>MKLDIKKTFSNRSDRVKGIDFHPTEPWVLTTLYSGRVEIWNYETQVEVRSIQVTETPVRAGKFIARKNWIIVGSDDFRIRVFNYNTGEKVVDFEAHPDYIRSIAVHPTKPYVLSGSDDLTVKLWNWENNWALEQTFEGHEHFVMCVAFNPKDPSTFASGCLDRTVKVWSLGQSTPNFTLTTGQERGVNYVDYYPLPDKPYMITASDDLTIKIWDYQTKSCVATLEGHMSNVSFAVFHPTL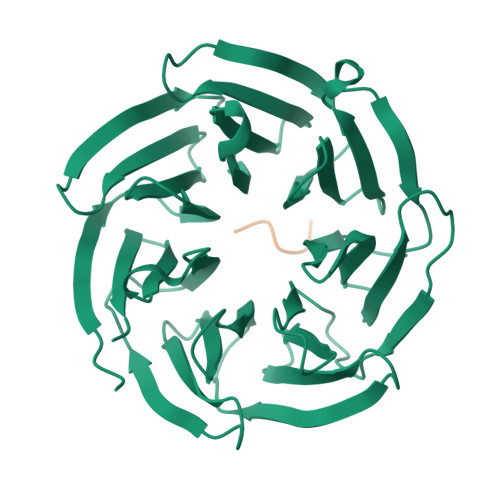PIIISGSEDGTLKIWNSSTYKVEKTLNVGLERSWCIATHPTGRKNYIASGFDNGFTVLSLG[2x];>KSHQE[2x]> MRRFGSKFASGLASRCALACPLASAATAPAGASTTSSTSSAQKSFFKTTEMIGYVHSIDGTIATLIPAPGNPGVAYNTIIQIQVSPTTFAAGLVFNLEKDGRIGIILMDNITEVQSGQKVMATGQLLHIPVGAGVLGKVVNPLGHEVPVGLVTRSRRLLDSTLGKVDTGAPNIVSRSPVNYNLLTGFKAVDTMIPIGRGQRELIVGDRQTGKTSIAVSTIINQVRINQQILSKNAVISIYVSIGQRCSNVARIHRLLQSYGALRYTTVMAATAAEPAGLQYLAPYA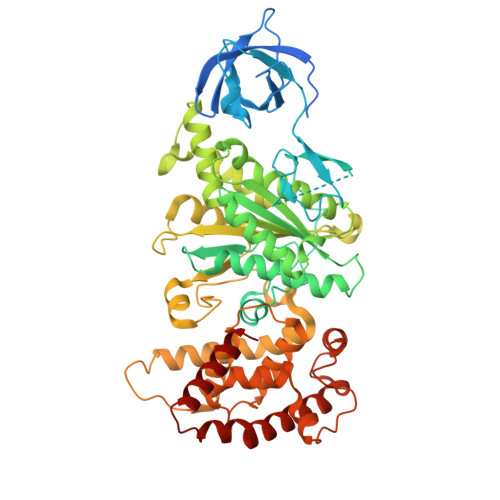GVTMGEYFMNRGRHCLCVYDDLSKQAVAYRQISLLLRRPPGREAYPGDVFYLHSRLLERAAMLSPGKGGGSVTALPIVETLSNDVTAYIVTNVISITDGQIYLDTKLFTGGQRPAVNIGLSVSRVGSSAQNAAMKGVAGKLKGILAEYRKLAADSVGGQQVQTIPMIRGARFVALFNQKQPSYFMNAIVSLYACLNGYLDDVKVQYVKFYEYLLVHRDLGIMYGTAKNKFFYMYVQELNYLIRFFTLNSPILHGELEEMLKQHTHLFLQHYQSKMNAIKSEKDVKALKNLLYSCKRAV(2-AMINOOXY-ETHYL)-[5-(6-AMINO-PURIN-9-YL)-3,4-DIHYDROXY-TETRAHYDRO-FURAN-2-YLMETHYL]-METHYL-SULFONIUM 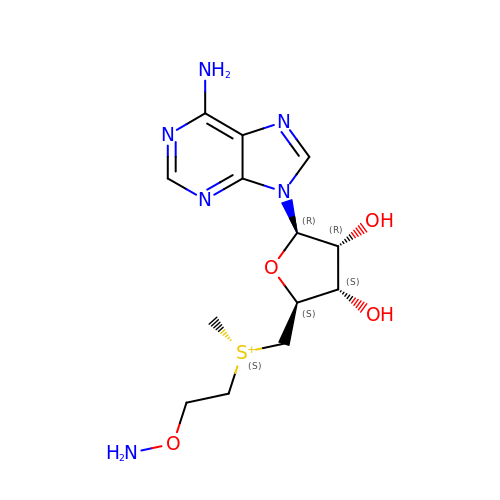| C13 H21 N6 O4 S | RMAOLICYOBWFLA-OCVRIJAPSA-N> GMEGAGQMAELPTHYGTIIKTLRKYMKLTQSKLSER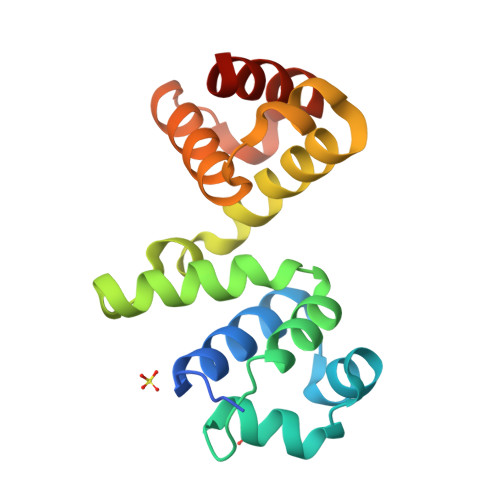TGFSQNTISNHENGNRNIGVNEIEIYGKGLGIPSYILHRISDEFKEKGYSPTLNDFGKFDKMYSYVNKAYYNDGDIYYSSYDLYDETIKLLELLKESKINVNDIDYDYVLKLYKQILSTDT~{N}-[4-methyl-3-[(1-methyl-6-pyridin-3-yl-pyrazolo[3,4-d]pyrimidin-4-yl)amino]phenyl]-3-(trifluoromethyl)benzamide | C26 H20 F3 N7 O | 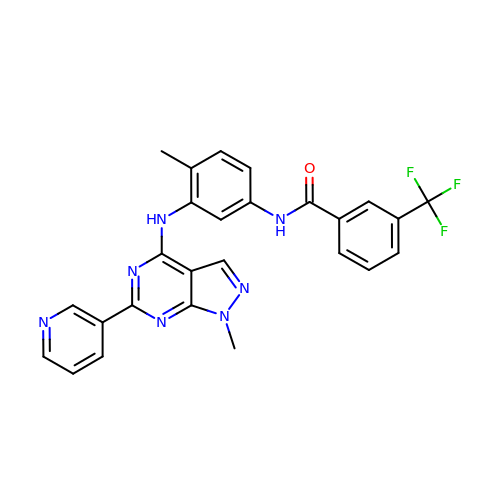QPABVIZUHZJQCR-UHFFFAOYSA-N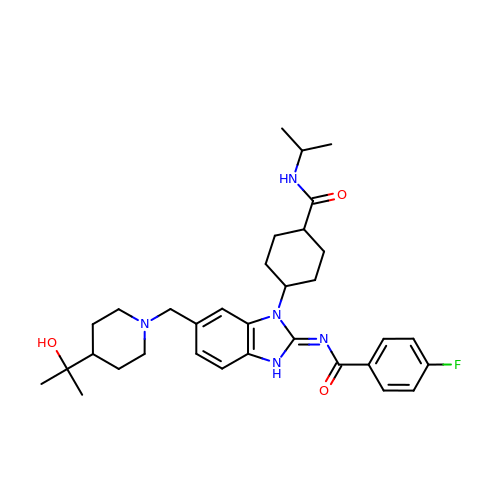4-fluoro-N-{(2E)-6-{[4-(2-hydroxypropan-2-yl)piperidin-1-yl]methyl}-1-[cis-4-(propan-2-ylcarbamoyl)cyclohexyl]-1,3-dihydro-2H-benzimidazol-2-ylidene}benzamide | C33 H44 F N5 O3 | WSTUJEXAPHIEIM-FEGDYQJNSA-N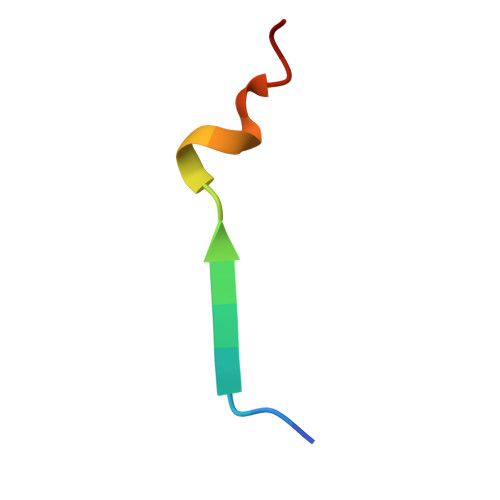> RRRTGTYGVLAAWRRL>AEPQPPSGGLTDEAALSCCSDADPSTKDFLLQQTMLRVKDPKKSLDFYTRVLGMTLIQKCDFPIMKFSLYFLAYEDKNDIPKEKDEKIAWALSRKATLELTHNWGTEDDETQSYHNGNSDPRGFGHIGIAVPDVYSACKRF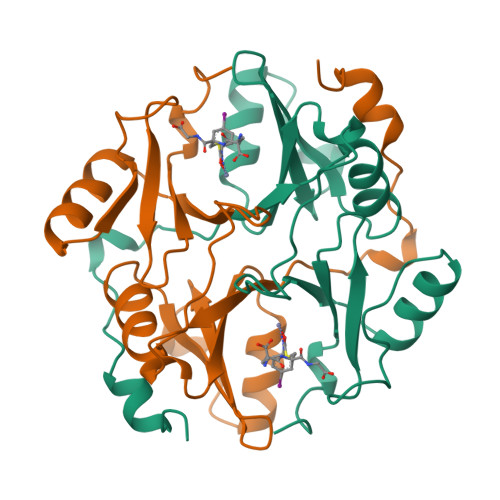EELGVKFVKKPDDGKMKGLAFIQDPDGYWIEILNPNKMATLM[2x]> GAMAAPLVTSVTETKELRGLNLIAAHSHIRGLGVDADTLEPRPSSQGLVGQEKARKAAAVVLEMIKQGKIAGRAVLIAGPPSTGKTAIAMGMAQSLGQDVPFTTLAASEIFSLEMSKTEALTQAFRKSIGVRIKEESEIMEGEVVEIQIDRSVTGGAKQGKLTIKTTDMEAIYDMGSKM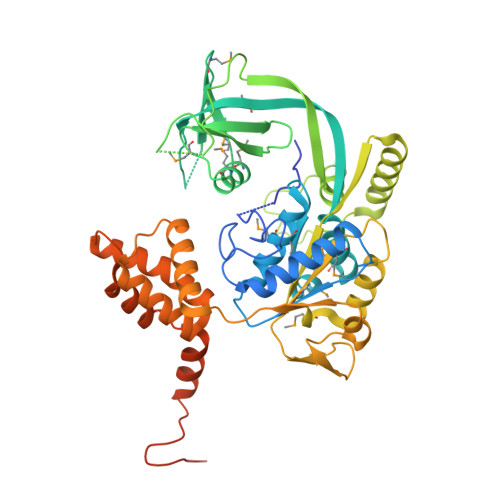IDAMTKERVMAGDIISIDKSSGKITKLGRSYARSRDYDAMGVDTKFLQCPEGELQKRKEVVHTVSLHEIDVINSRTQGFLALFSGDTGEIRSEIRDQINTKVAEWKEEGKAEIVPGVLFIDEVHMLDIECFSYINRALESDLAPIVIMASNRGVSRIRGTDYKSPHGLPLDFLDRVVIINTHPYTPDELRQILSIRAQEEEVDLTPDALALLTKIGQEAGLRYASNLITTSQLIAAKRRAKQVGVEDVQRSFKLFYDPARSVRFVQESEKRLIGNDGVVDFSYQGAAEAAAPTLPAAAPVDPVGGEKMDMS>[12x]STRFTEEYQLFEELGKGAFSVVRRCVKVLAGQEYAAKIINTKKLSARDHQKLEREARICRLLKHPNIVRLHDSISEEGHHYLIFDLVTGGELFEDIVAREYYSEADASHCIQQILEAVLHCHQMGVVHRDLKPENLLLASKLKGAAVKLADFGLAIEVEGEQQAWFGFAGTPGYLSPEVLRKDPYGKPVDLWACGVILYILLVGYPPFWDEDQHRLYQQIKAGAYDFPSPEWDTVTPEAKDLINKMLTINPSKRITAAEALKHPWISHRSTVASCMHRQETVDCLKKFNARRKLKGAILTTMLATRNFSGGKSGGNKKSDGVKESSESTNTTIEDEDTKVRKQEIIKVTEQLIEAISNGDFESYTKMCDPGMTAFEPEALGNLVEGLDFHRFYFENLWSRNSKPVHTTILNPHIHLMGDESACIAYIRITQYLDAGGIPRTAQSEETRVWHRRDGKWQIV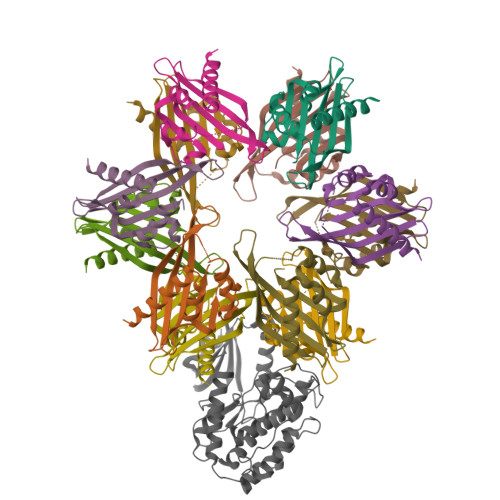HFHRSGAPSVLPH;> STRFTEEYQLFEELGKGAFSVVRRCVKVLAGQEYAAMIINTKKLSARDHQKLEREARICRLLKHPNIVRLHDSISEEGHHYLIFDLVTGGELFEDIVAREYYSEADASHCIQQILEAVLHCHQMGVVHRNLKPENLLLASKLKGAAVKLADFGLAIEVEGEQQAWFGFAGTPGYLSPEVLRKDPYGKPVDLWACGVILYILLVGYPPFWDEDQHRLYQQIKAGAYDFPSPEWDTVTPEAKDLINKMLTINPSKRITAAEALKHPWISHRSTVASCMHRQETVDCLKKFNARRKLKGAILTTMLATRNFSGGKSGGNKKSDGVKESSESTNTTIEDEDTKVRKQEIIKVTEQLIEAISNGDFESYTKMCDPGMTAFEPEALGNLVEGLDFHRFYFENLWSRNSKPVHTTILNPHIHLMGDESACIAYIRITQYLDAGGIPRTAQSEETRVWHRRDGKWQIVHFHRSGAPSVLPH> AMFLQRPKPYSDESLESFFIRVANKNGYGDVHRFLEATKRFLQDIDHNGYQTFPTDITRINPYSAKNSSSARTASFLKLAQLTFNEPPELLGLAINRTNMKYSPSTSAVVRGAEVFPRSLLRTHSIPCCPLCLRENGYASYLWHFQGYEYCHSHNVPLITTCSCGKEFDYRVSEA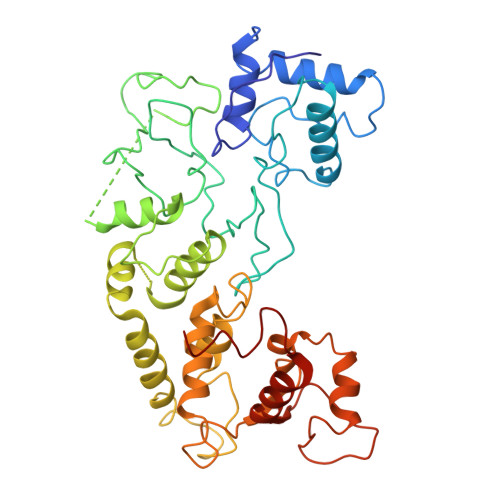ACTVSNWLAGHESKPLPNLPKSYRWGLVHWWMGIKDDHFSFVQFFSNWPRSFHSIIEDEVEFNLEHAVVSTSELRLKDLLGRLFFGSIRLPERNLQHNIILGELLCYLENRLWQDKGLIANLKMNALEATVMLNCSLDQIASMVEQRILKPNAAAAAAAAADVTDYLFHFGDIFCLWLAAFQSDEFNRSFYVSR> MSMLKREDWYDLTRTTNWTPKYVTENELFPEEMSGARGISMEAWEKYDEPYKITYPEYVSIQREKDSGAYSIKAALERDGFVDRADPGWVSTMQLHFGAIALEEYAASTAEARMARFAKAPGNRNMATFGMMDENRHGQIQLYFPYANVKRSRKWDWAHKAIHTNEWAAIAARSFFDDMMMTRDSVAVSIMLTFAFETGFSNMQFLGLAADAAEAGDHTFASLISSIQTDESRHAQQGGPSLKILVENGKKDEAQQMVDVAIWRSWKLFSVLTGPIMDYYTPLESRNQSFKEFMLEWIVAQFERQLLDLGLDKPWYWDQFMQDLDETHHGMHLGVWYWRPTVWWDPAAGVSPEEREWLEEKYPGWNDTWGQCWDVITDNLVNGKPELTVPETLPTICNMCNLPIAHTPGNKWNVKDYQLEYEGRLYHFGSEADRWCFQIDPERYENHTNLVDRFLKGEIQPADLAGALMYMSLEPGVMGDDAHDYEWVKAYQKKTNAA;> MSEQQPEALKPLKTWSHLAGNRRRPSEYEVVSTNLHYFTDNPERPWELDSNLPMQTWYKKYCFDSPLKHDDWNAFRDPDQLVYRTYNLLQDGQESYV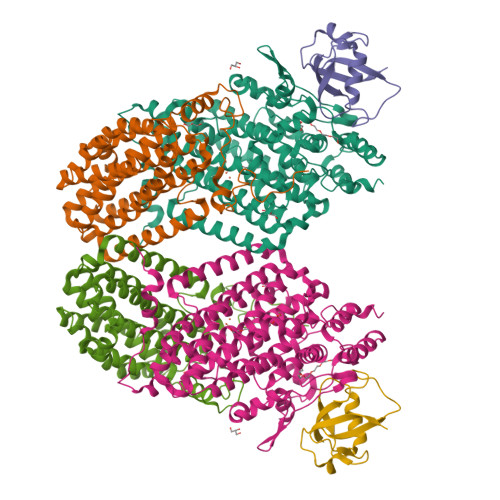QGLFDQLNDRGHDQMLTREWVETLARFYTPARYLFHALQMGSVYIHQIAPASTITNCATYETADHLRWLTHTAYRTRELANCYPDVGFGKRERDVWENDPAWQGFRELIEKALIAWDWGEAFTAINLVTKPAVEEALLQQLGSLAQSEGDTLLGLLAQAQKRDAERHRRWSSALVKMALEKEGNREVLQKWVAKWEPLADKAIEAYCSALPDGENAIVEAKSASRYVRQMMGL;> MATFPIMSNFERDFVIQLVPVDTEDTMDQVAEKCAYHSINRRVHPQPEKILRVRRHEDGTLFPRGMIVSDAGLRPTETLDIIFMDN>ETEKLIRMKDEELRRMQEMLQRMKQQ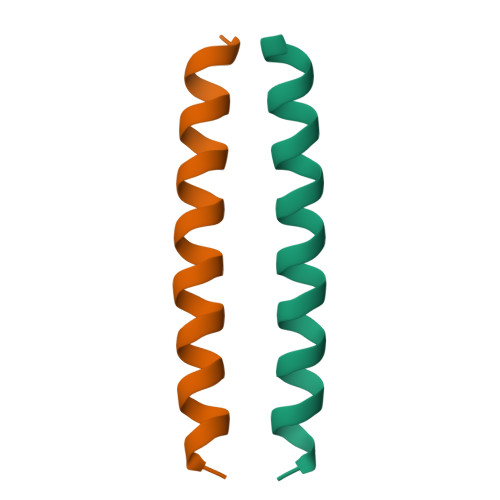MQDQ[2x]>[4x]MKGFAMLSIGKVGWIEKEKPAPGPFDAIVRPLAVAPCTSDIHTVFEGAIGERHNMILGHEAVGEVVEVGSEVKDFKPGDRVVVPAITPDWRTSEVQRGYHQHSGGMLAGWKFSNVKDGVFGEFFHVNDADMNLAHLPKEIPLEAAVMIPDMMTTGFHGAELADIELGATVAVLGIGPVGLMAVAGAKLRGAGRIIAVGSRPVCVDAAKYYGATDIVNYKDGPIESQIMNLTEGKGVDAAIIAGGNADI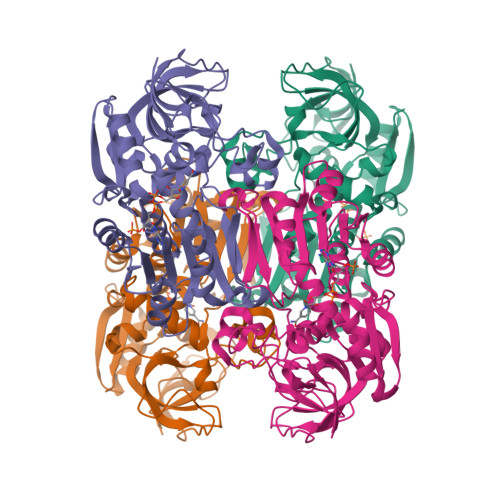MATAVKIVKPGGTIANVNYFGEGEVLDVPRLEWGCGMAHKTIKGGLCPGGRLRMERLIDLVFYKRVDPSKLVTHVFRGFDNIEKAFMLMKDKPKDLIKPVVILA6-[(Z)-2-{3-[(1S,5S,6S)-3-amino-5-methyl-1-(morpholine-4-carbonyl)-2-thia-4-azabicyclo[4.1.0]hept-3-en-5-yl]-4-fluorophenyl}-1-fluoroethenyl]pyridine-3-carbonitrile 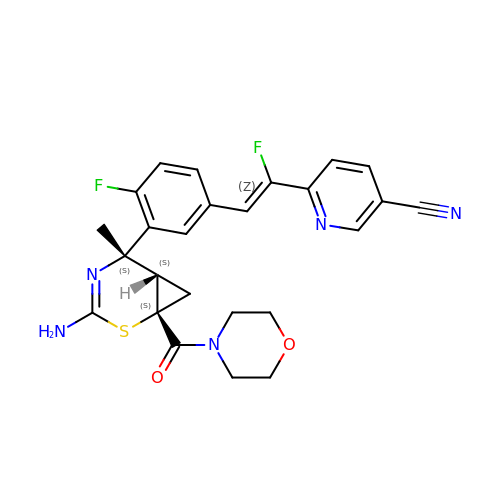| C25 H23 F2 N5 O2 S | VZHFJCNPAIRJSA-MYMUPAQMSA-N>[2x]GSKPPSGSPETGAGAGTVATTPASSPVTLAETGSTLLYPLFNLWGPAFHERYPNVTITAQGTGSGAGIAQAAAGTVNIGASDAYLSEGDMAAHKGLMNIALAISAQQVNYNLPGVSEHLK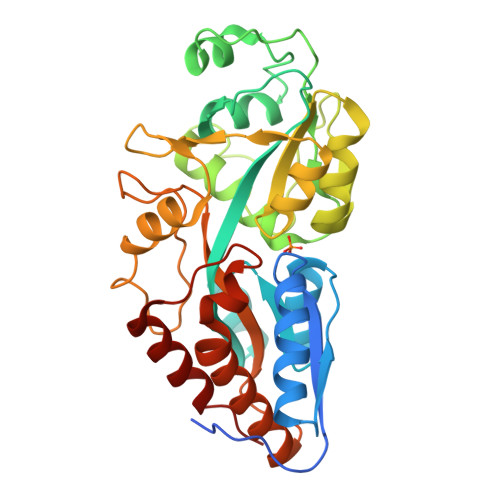LNGKVLAAMYQGTIKTWDDPQIAALNPGVNLPGTAVVPLHRSDGSGDTFLFTQYLSKQDPEGWGKSPGFGTTVDFPAVPGALGENGNGGMVTGCAETPGCVAYIGISFLDQASQRGLGEAQLGNSSGNFLLPDAQSIQAAAAGFASKTPANQAISMIDGPAPDGYPIINYEYAIVNNRQKDAATAQTLQAFLHWAITDGNKASFLDQVHFQPLPPAVVKLSDALIATISS>[4x]MSDSHHKPVWDRTHHAKMATGIGDPQCFKGMAGKSKFNVGDRVRIKDLPDLFYTRTMTYTRGATGTIVRLVYESPAAEDEAFGNEENVEWFYSIVFAQKDLWPEYSDTFANDTLETEIPERYLEKA;>[4x]MSSSIREEVHRHLGTVALMQPALHQQTHAPAPTEITHTLFRAYTRVPHDVGGEADVPIEYHEKEEEIWELNTFATCECLAWRGVWTAEERRRKQNCDVGQTVYLGMPYYGRWLLTAARILVDKQFVTLTELHNKIVEMRERVASGQGLGEYLPPKAK;>MSADHDHDHDHDHDHKPAPMVEEVSDFEILEMAVRELAIEKGLFSAEDHRVWKDYVHTLGPLPAARLVAKAWLDPEYKKLCIEDGVEASKAVGVNWVTSPPTQFGTPSDYCNLRVLADSPTLKHVVVCTLCSCYPRPILGQSPE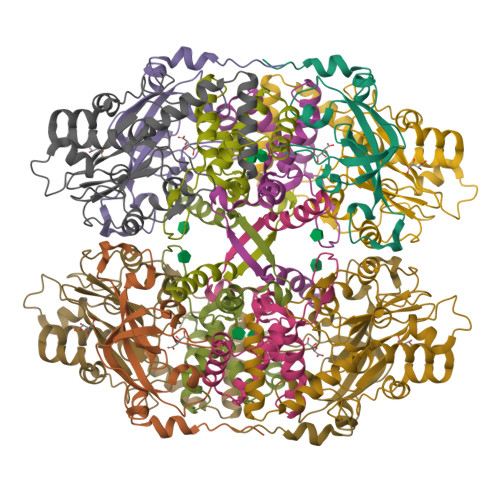WYRSPNYRRRLVRWPRQVLAEFGLQLPSEVQIRVADSNQKTRYIVMPVRPEGTDGWTEDQLAEIVTRDCLIGVAVPKPGITVNAKRPVLKANRPVHHDH[4x]>GSGSGSCVKWFIYGVIAVYICYTLIVHKRYQEKEELTSSVRVTLKGVAHVDRIWDAAEYTIPTQTRDSFFVMTNIIRTENQIQKTCPEYPTAKAICSSDKSCAKGIVDVHSNGVQTGKCVHYNITHKTCEIKAWCPVQGEERPPVPAVLRSSEDFTVFIKNNIHFPTFQYTVQNISPKLNTSCKFNKVTAPLCPIFRLGDILQEAKENFSEMAVKGGIIAIEIKWDCDLDSWSYYCSPEYSFRRLDDKTRTQYPGFSIRFARHYKLPDGTEQRTLFKAYGIRFDVLVFGMGGQFKLIELFTFIGSTIAYFGLAVTIIEMCFHLYNLE[3x]

The vertebrate P2X receptors include seven subtypes (P2X1–P2X7) that form homo- or hetero-trimers and are involved in diverse physiological processes, such as muscle contraction, pain sensation, inflammation, and perception. Each subunit of the P2X receptor is composed of the large extracellular domain that contains the ATP and other ligand binding sites, the two transmembrane helices that form a non-selective cation pore, and the intracellular N- and C-termini that modulate channel gating. Among the P2X receptor subtypes, the P2X7 receptors have a unique, long intracellular C-terminus with protein binding, phosphorylation, and lipid recognition sites. Therefore, P2X7 receptors play a crucial role in inflammation, immunity, neurological function, and apoptosis.

Here, we report the crystal structure of the chicken P2X7 receptor in complex with TNP-ATP. The ckP2X7cryst construct lacks the regions encoding 27 N-terminal and 214 C-terminal residues, which were predicted to be structurally disordered, and includes the mutation of Asn190 to exclude a putative glycosylation site. The crystals of ckP2X7cryst in complex with TNP-ATP were obtained by the vapor diffusion method, and diffracted X-rays to 3.1 Å resolution. The overall assembly and subunit folding of ckP2X7cryst are consistent with those of the previously determined P2X structures, sharing the chalice-like trimeric architecture with a large hydrophilic extracellular domain, two transmembrane helices, and intracellular termini, resembling the shape of a dolphin. In the TNP-ATP-bound ckP2X7 structure, the TNP-ATP molecule is located in the ATP binding pocket, and thus interacts with the head, upper body, right flipper, and left flipper domains from one subunit, and the lower body and dorsal fin domains from the neighboring subunit. First, the adenine ring of TNP-ATP adopts a similar orientation to that observed in the previously reported ATP-bound P2X structures, and thus forms hydrogen bonds with the side chains of the highly conserved ckThr177 and the main chain carbonyl groups of ckThr64 and ckThr177. Next, in the TNP-ATP-bound ckP2X7 structure, the phosphate groups of TNP-ATP adopt a totally extended conformation, whereas the phosphate groups of ATP in the previous structures form a bent, “U-shaped” conformation. The different orientation of the ribose group also changes that of the trinitrophenyl group: the trinitrophenyl group in the TNP-ATP-bound ckP2X7 structure contacts the head and dorsal fin domains, forming three hydrogen bonds with the side chains of ckLys66, ckThr112, and ckThr202. Consistently, the ion-conducting pore is still closed in the TNP-ATP-bound ckP2X7 structure. This “incompletely activated” conformation of the TNP-ATP-bound ckP2X7 structure is apparently due to the insertion of the trinitrophenyl group between the head and dorsal fin domains, which prevents the complete cleft closure motion in the ATP binding pocket.>SKNKEDKRNAEYRLAFEQLNFVGADSKTPILKSFIEDKGTRIDEITFESMIPIETWKSYIPQLQTSLNISIISIEQGASKRIVIIKSMAGDAKIPKYLPWDDKYIEEQEGVVVVGQTFSGNIKIDLNKSPHILSAGETGSGKSVILRCILWQLLKQGAIAYMVDFKGGVEFGLEYEKVGQVITEVDAAEKLFKYLVDENAKRLKLLRESGSKNIGEYNKKFEGEELKRIIVVIDELAELMDKTGVDDETRAKLVRIEGYTSTL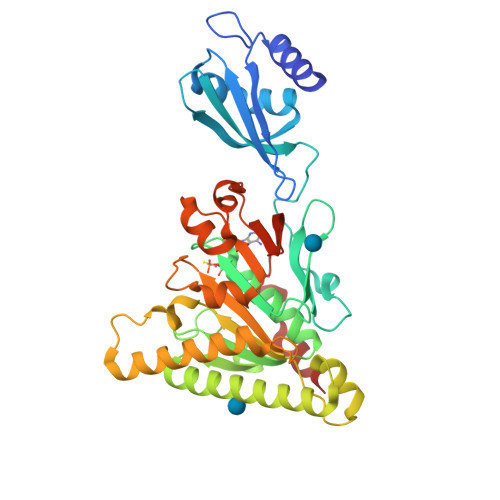ARLSRATGINLCIGVQRPDAKVITGQIKNNVPVRICGRFADSKASEIVLSNTKAKDLPEVKGRFLFKLGADTVQFQAFYFDDDKHFIPNKILKLRK[2x]>GPLGSMSEEQVAQDTEEVFRSYVFYRHQQEQEAEGVAAPADPEMVTLPLQPSSTMGQVGRQLAIIGDDINRRYDSEFQTMLQHLQPTAENAYEYFTKIATSLFESGINWGRVVALLGFGYRLALHVYQHGLTGFLGQVTRFVVDFMLHHSIARWIAQRGGWVAALNLGNG[2x];>SRIISRIAQELRRXGDEFNATYA[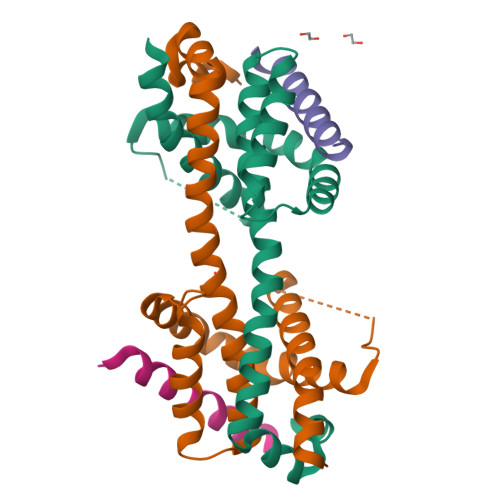2x]> SLNINDALTSILASKKYRALCPDTVRRILTEEWGRHKSPKQTVEAARTRLHGICGAYVTPESLKAAAAALSAGDVKKALSLHAS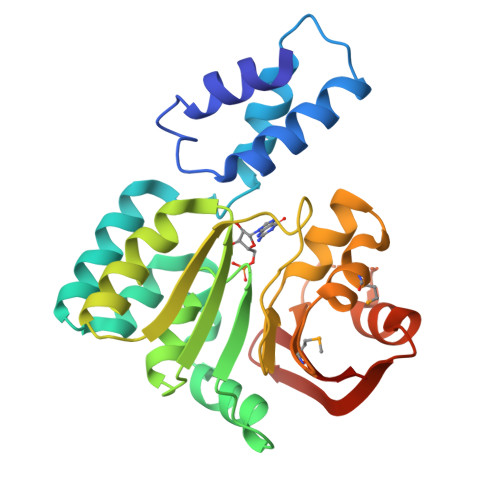TKERLAELDTLYDFIFSAETPRRVLDIACGLNPLALYERGIASVWGCDIHQGLGDVITPFAREKDWDFTFALQDVLCAPPAEAGDLALIFKLLPLLEREQAGSAMALLQSLNTPRMAVSFPTRSLGGRGKGMEANYAAWFEGGLPAEFEIEDKKTIGTELIYLIKKNG>EYNAPSEIKYIDVVNTYDLEEEASKVVPHGGFNYIAGASGDEWTKRANDRAWKHKLLYPRLAQDVEAPDTSTEILGHKIKAPFIMAPIAAHGLAHTTKEAGTARAVSEFGTIMSISAYSGATFEEISEGLNGGPRWFQIYMAKDDQQNRDILDEAKSDGATAIILTADSTVSGNRDRDVKNKFVYPFGMPIVQRYLRGTAEGMSLNNIYGASKQKISPRDIEEIAAHSGLPVFVKGIQHPEDADMAIKRGASGIWVSNHGARQLYEAPGSFDTLPAIAERVNKRVPIVFDSGVRRGEHVAKALASGADVVALGRPVLFGLALGGWQGAYSVLDYFQKDLTRVMQLTGSQNVEDLKGLDLFDNPYGYEYEYNAPSEIKYIDVVNTYDLEEEASKVVPHGGFNYIAGASGDEWTKRANDRAWKHKLLYPRLAQDVEAPDTSTEILGHKIKAPFIMAPIAAHGLAHTTKEAGTARAVSEFGTIMSISAYSGATFEEISEGLNGGPRWFQIYMAKDDQQNRDILDEAKSDGATAIILTADSTVSGNRDRDVKNKFVYPFGMPIVQRYLRGTAEGMSLNNIYGASKQKISPRDIEEIAAHSGLPVFVKGIQHPEDADMAIKRGASGIWVSNHGARQLYEAPGSFDTLPAIAERVNKRVPIVFDSGVRRGEHVAKALASGADVVALGRPVLFGLALGGWQGAYSVLDYFQKDLTRVMQLTGSQNVEDL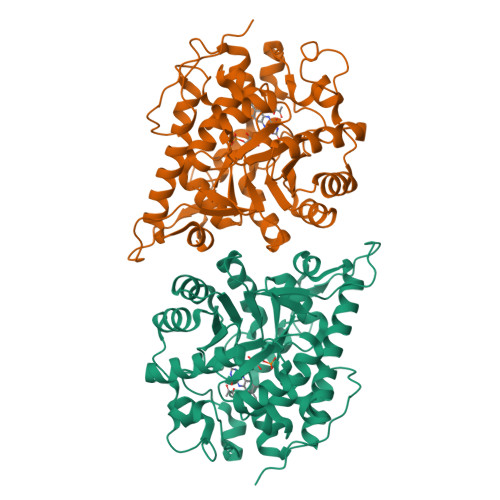KGLDLFDNPYGYEY[2x]>[2x]GAPATVTEQGEDITSKKDRGVLKIVKRVGNGEETPMIGDKVYVHYKGK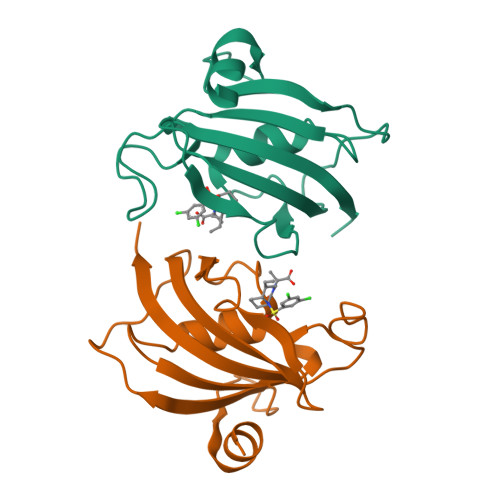LSNGKKFDSSHDRNEPFVFSLGKGQVIKAWDIGVATMKKGEICHLLCKPEYAYGSAGSLPKIPSNATLFFEIELLDFKGE> MSADSSPLVGSTPTGYGTLTIGTSIDPLSSSVSSVRLSGYCGSPWRVIGYHVVVWMMAGIPLLLFRWKPLWGVRLRLRPCNLAHAETLVIEIRDKEDSSWQLFTVQVQTEAIGEGSLEPSPQSQAEDGRSQAAVGAVPEGAWKDTAQLHKSEEAKRVLRYYLFQGQRYIWIETQQAFYQVSLLDHGRSCDDVHRSRHGLSLQDQMVRKAIYGPNVISIPVKSYPQLLVDEALNPYYGFQAFSIALWLADHYYWYALCIFLISSISICLSLYKTRKQSQTLRDMVKLSMRVCVCRPGGEEEWVDSSELVPGDCLVLPQEGGLMPCDAALVAGECMVNESSLTGESIPVLKTALPEGLGPYCAETHRRHTLFCGTLILQARAYVGPHVLAVVTRTGFCTAKGGLVSSILHPRPINFKFYKHSMKFVAALSVLALLGTIYSIFILYRNRVPLNEIVIRALDLVTVVVPPALPAAMTVCTLYAQSRLRRQGIFCIHPLRINLGGKLQLVCFDKTGTLTEDGLDVMGVVPLKGQAFLPLVPEPRRLPVGPLLRALATCHALSRLQDTPVGDPMDLKMVESTGWVLEEEPAADSAFGTQVLAVMRPPLWEPQLQAMEEPPVPVSVLHRFPFSSALQRMSVVVAWPGATQPEAYVKGSPELVAGLCNPETVPTDFAQMLQSYTAAGYRVVALASKPLPTVPSLEAAQQLTRDTVEGDLSLLGLLVMRNLLKPQTTPVIQALRRTRIRAVMVTGDNLQTAVTVARGCGMVAPQEHLIIVHATHPERGQPASLEFLPMESPTAVNGVKDPDQAASYTVEPDPRSRHLALSGPTFGIIVKHFPKLLPKVLVQGTVFARMAPEQKTELVCELQKLQYCVGMCGDGANDCGALKAADVGISLSQAEASVVSPFTSSMASIECVPMVIREGRCSLDTSFSVFKYMALYSL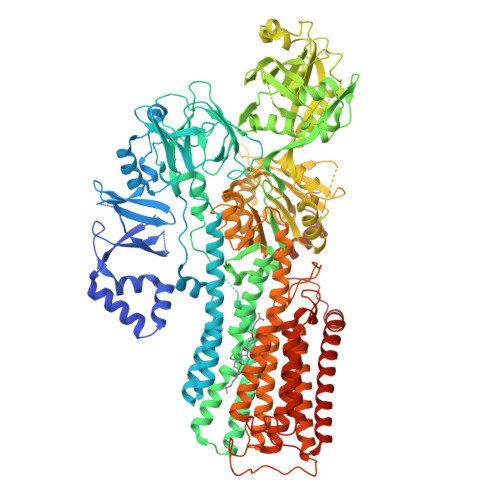TQFISVLILYTINTNLGDLQFLAIDLVITTTVAVLMSRTGPALVLGRVRPPGALLSVPVLSSLLLQMVLVTGVQLGGYFLTLAQPWFVPLNRTVAAPDNLPNYENTVVFSLSSFQYLILAAAVSKGAPFRRPLYTNVPFLVALALLSSVLVGLVLVPGLLQGPLALRNITDTGFKLLLLGLVTLNFVGAFMLESVLDQCLPACLRRLRPKRASKKRFKQLERELAEQPWPPLPAGPLR>[2x]PRLYFENRSKFIQDQKDKGINPYPHKFERTISIPEFIEKYKDLGNGEHLEDTILNITGRIMRVSASGQKLRFFDLVGDGEKIQVLANYSFHNHEKGNFAECYDKIRRGDIVGIVGFPGKSKKGELSIFPKETILLSACLHMLPMKYGLKDTEIRYRQRYLDLLINESSRHTFVTRTKIINFLRNFLNERGFFEVETPMMNLIAGGANARPFITHHNDLDLDLYLRIATELPLKMLIVGGIDKVYEIGKVFRNEGIDNTHNPEFTSCEFYWAYADYNDLIKWSEDFFSQLVYHLFGTYKISYNKDGPENQPIEIDFTPPYPKVSIVEEIEKVTNTILEQPFDSNETIEKMINIIKEHKIELPNPPTAAKLLDQLASHFIENKYNDKPFFIVEHPQIMSPLAKYHRTKPGLTERLEMFICGKEVLNAYTELNDPFKQKECFKLQQKDREKGDTEAAQLDSAFCTSLEYGLPPTGGLGLGIDRITMFLTNKNSIKDVILFPTMRPA

Aminoacyl-tRNA synthetases catalyze aminoacylation of tRNAs with their cognate amino acids in two stages. First, the amino acid is activated by ATP to yield the AMP-activated amino acid, with loss of pyrophosphate, followed by transfer of the amino acid onto the tRNA. Malaria parasite genomes encode two different lysyl-tRNA synthetases (KRSs) that play a role in translation in either the cytoplasm (PfKRS1) or in the apicoplast (PfKRS2), while Cryptosporidium parasites and humans encode one copy. We present a selective inhibitor of both Plasmodium and Cryptosporidium lysyl-tRNA synthetase capable of clearing parasites from mouse models of malaria and cryptosporidiosis infection.

Addition of a fluorine in the phenyl ring at C-6 blocked hydroxylation at the phenyl ring of the chromone (compound 3), and introduction of a hydroxyl at the bridgehead of the cyclohexyl substituent was tolerated without loss of potency, while reducing lipophilicity and intrinsic clearance (compound 4). The cocomplex of 4 bound to PfKRS1 showed that the ligand retained the binding mode of 2, conserving key H-bonds from the core scaffold to the protein. The addition of the 6F atom did not afford new interactions with the protein or ordered solvent. The bridgehead hydroxyl was close to the side chain of E500, forming a weak interaction (3.4 Å) and interacting with the ordered water network.4-[2-(1,1,3,3-tetramethyl-2,3-dihydro-1H-inden-5-yl)-1,3-dioxolan-2-yl]benzoic 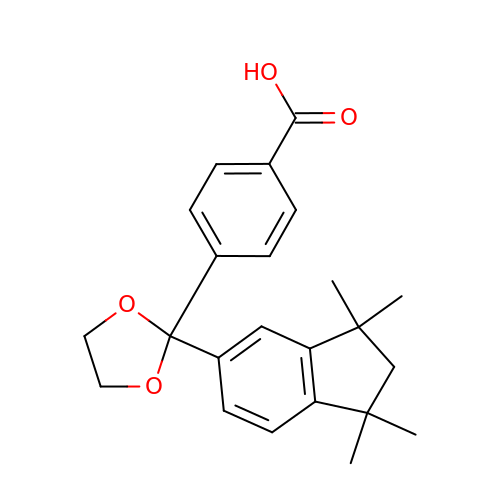acid | C23 H26 O4 | ISZBCQLHSNHWLM-UHFFFAOYSA-N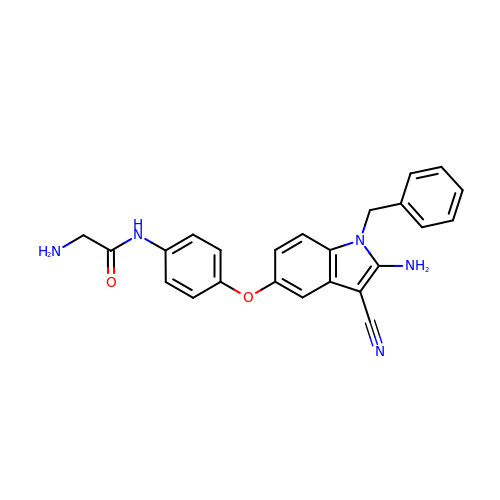2-amino-N-[4-(2-amino-1-benzyl-3-cyano-indol-5-yl)oxyphenyl]acetamide | C24 H21 N5 O2 | RVTAACJVJXEMFR-UHFFFAOYSA-N> ACGTCT;> GAACGACAGAGACGTCGACTC;> TC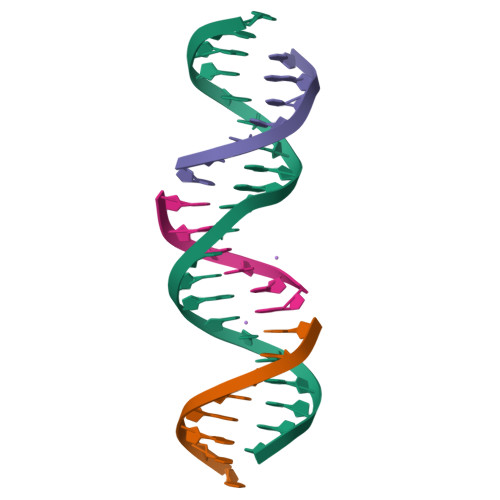GAGTCG;> CTGTCGT>[2x]MARLLTNKNHKVEVQLSADGTEFDSTTFVKELPAEEKLSIATDYSNDYKKH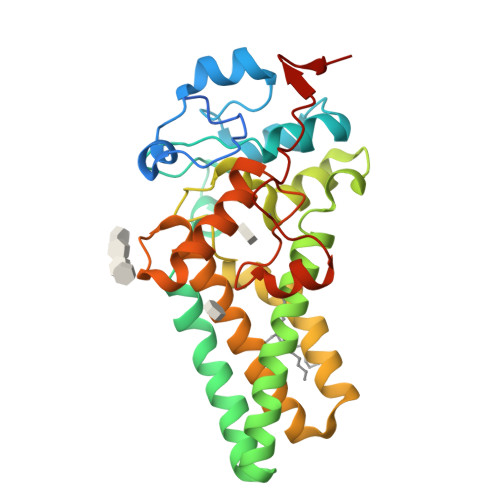KFLDLNRPLLMQILRSDFKKDFYVDQIHRPRHYGKGSAPLFGNFLEPLTKTAWWVVPVAWLPVVVYHMGVALKNMNQLFACFLFCVGVFVWTLIEYGLHRFLFHFDDWLPESNIAFATHFLLHGCHHYLPMDKYRLVMPPTLFVILCAPFYKLVFALLPLYWAYAGFAGGLFGYVCYDECHFFLHHSKLPPFMRKLKKYHLEHHYKNYQLGFGVTSWFWDEVFGTYLGPDAPLSKMKYESGLEVLFQ2-bromo-4-tert-butyl-6-{[(3-phenylpropyl)amino]methyl}phenol | C20 H26 Br N O | 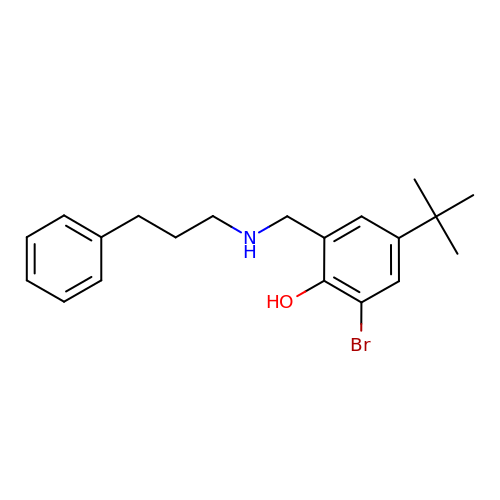LIVFSGNFBWATFT-UHFFFAOYSA-N> MKTTTPLVHVASVEKGRSYEDFQKVYNAIALKLREDDEYDNYIGYGPVLVRLAWHISGTWDKHDNTGGSYGGTYRFKKEFNDPSNAGLQNGFKFLEPIHKEFPWISSGDLFSLGGVTAVQEMQGPKIPWRCGRVDTPEDTTPDNGRLPDADKDAGYVRTFFQRLNMNDREVVALMGAHALGKTHLKNSGYEGPWGAANNVFTNEFYLNLLNEDWKLEKNDANNEQWDSK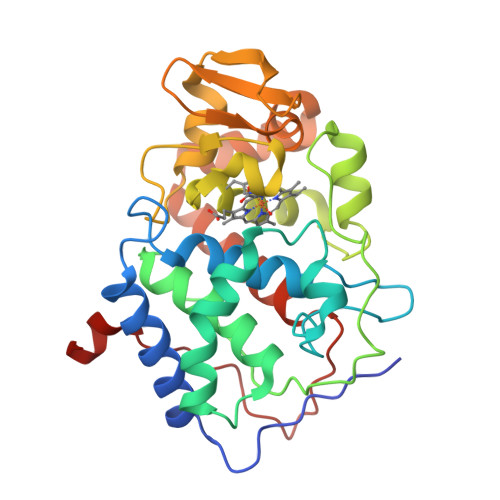SGYMMLPTDYSLIQDPKYLSIVKEYANDQDKFFKDFSKAFEKLLENGITFPKDAPSPFIFKTLEEQGL>HHHHHHMAKKVNWYVSCSPRSPEKIQPELKVLANFEGSYWKGVKGYKAQEAFAKELAALPQFLGTTYKKEAAFSTRDRVAPMKTYGFVFVDEEGYLRITEAGKMLANNRRPKDVFLKQLVKWQYPSFQHKGKEYPEEEWSINPLVFVLSLLKKVGGLSKLDIAMFCLTATNNNQVDEIAEEIMQFRNEREKIKGQNKKLEFTENYFFKRFEKIYGNVGKIREGKSDSSHKSKIETKMRNARDVADATTRYFRYTGLFVARGNQLVLNPEKSDLIDEIISSSKVVKNYTRVEEFHEYYGNPSLPQFSFETKEQLLDLAHRIRDENTRLAEQLVEHFPNVKVEIQVLEDIYNSLNKKVDVETLKDVIYHAKELQLELKKKKLQADFNDPRQLEEVIDLLEVYHEKKNVIEEKIKARFIANKNTVFEWLTWNGFIILGNALEYKNNFVIDEELQPVTHAAGNQPAMEIIYEDFIVLGEVTTSKGATQFKMESEPVTRHYLNKKKELEKQGVEKELYCLFIAPEINKNTFEEFMKYNIVQNTRIIPLSLKQFNMLLMVQKKLIEKGR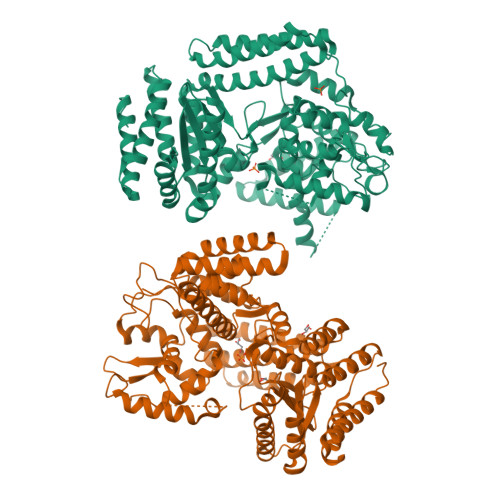RLSSYDIKNLMVSLYRTTIECERKYTQIKAGLEETLNNWVVDKEVRF[2x]>MINNKLLNIETMKKLFLFFYLSVVSIAAFAAEQFVIFTPAGNHFPLVANGVPCPIYIDSSEDKGVMIAAGNLQQDILQVCGKKPELLTSTSSKRCIIAGTYGTPFIKKLMSAGKIDKKELDGKNEKYILQVIANPCEGIDEAVVIIGSDRRGTIYGIYELSEQMGVSPWYWWADVPVMKQANVYIKPGQYSDGEPAVTYRGIFLNDEAPCLTRWVKHTYGTNYGDHRFYARVCELILRLKGNFLWPAMWSWAFYADDPQNSKTASEMGVIIGTSHHEPMARNHQEWSRKRKEYGAWDYTTNQKVIDQFFREGIERMQGTEDIVTIGMRGDGDAAMSKSTNVKLLENVVKNQRKIIEEVTKRPAKETPQVWALYKEVLDYYDKGMRVPDDVIMLLCDDNWGNVCRLPNAKERKHPGGWGMYYHVDYVGAPRNSKWLNVTPIQNMWEQLQLTYDYGVEKLWILNVGDLKPMEYPITLFMDMAWNPKQFNVSNLLDHPRRFCAQQFGEDQADEAMRILNLYSKYNGRVTGEMLDRNTYNLETGEWKQVSDEYLKLEAEALRQYISLKPEYKDAYKQLILFPVQAMANLYEMYYAQAMNHKLYKENNPQANEWADKVEQAFARDKALSDDYNNIMSGGKWKNMMIQKHIGYTSWNDNFPADTLPKIYRIENPEKAVGGYVFTGQDGYIAIEAEHYYSAKAAPDTEWTVIPYMGRTLSGMALMPYTQPTDGASISYKIKLPKGIDKVTVHVIVKSTLAFHDRKGHEYSIGFEGGKDQTINFNHNLNELPENVYSIYYPTVARRIVEKKAKLNVPNTSDGMQTITFKPLDPGIVLEKLVVDYGGYKKSYLFMNESKSKRESR[2x]

Here we show that a dominant member of the human microbiota, Bacteroides ovatus, contains a GH115 enzyme, BoAgu115A, which displays glucuronoxylan α-(4-O-methyl)-glucuronidase activity. The enzyme is significantly more active against substrates in which the xylose decorated with GlcA/MeGlcA is flanked by one or more xylose residues. The crystal structure of BoAgu115A revealed a four-domain protein in which the active site, comprising a pocket that abuts a cleft-like structure, is housed in the second domain that adopts a TIM barrel-fold. The third domain, a five-helical bundle, and the C-terminal β-sandwich domain make inter-chain contacts leading to protein dimerization.

The crystal structure of the native BoAgu115A was solved by extending the phase information from an initial selenomethionine SAD at 3.0 Å to a native resolution of 2.65 Å, whereas the ligand structure of the enzyme was determined by molecular replacement at a resolution of 2.14 Å. Inspection of the surface of the BoAgu115A protomers revealed a cleft-like structure in the (β/α)8 domain that extends over the central β-barrel, on the opposite surface to the N-terminal domain. The center of the cleft, which may accommodate the xylan backbone, abuts onto a deep pocket that likely comprises the active site. The Oδ-2 of Asp-332 in the apo structure (the amino acid is not visible in the structure of the BoAgu115A-GlcA complex, discussed in detail below), is in an appropriate position to make polar contacts with O2 of GlcA, whereas Oδ-1 of Asp-206 forms a polar contact with O1 and may therefore act as the catalytic acid. Based on mutagenesis data the other carboxylate amino acids in the vicinity of the active site, Asp-332 and Glu-375, are candidate catalytic residues; the D332A and E375A mutations caused complete inactivation of the enzyme and a ∼5000-fold reduction in activity, respectively. It is evident, however, that the distance between Asp-332 and Glu-375 (in the apo structure) and the O1 of GlcA (in the structure of BoAgu115A in complex with GlcA); 5.4 Å and 11.8 Å, respectively, are greater than the normal ∼3.5 Å between the catalytic base and the anomeric carbon of the glycone sugar in inverting glycoside hydrolases. In enzymes and non-catalytic binding proteins that interact with glucuronic acid, arginines are often important specificity determinates, making bidentate hydrogen bonds/salt bridges with the carboxylate group. It is possible that in BoAgu115A Arg-328 contributes to substrate binding by also interacting with the carboxylate of the glucuronic acid substrate, a view supported by the observation that the R328A mutation caused ∼105-fold decrease in activity. Arg-328 (and Glu-375) in the apo structure, however, are too distant from the hub of the active site to play a direct role in enzyme function. Thus, for the arginine to contribute to substrate binding the loop containing this amino acid (and Asp-332) would be required to undergo a conformational change.Here, we study fold transition between distinct β-barrels by protein engineering and structural biology technique. Here, we discover that the previously reconstructed ancient DPBB sequence could also adopt a β-barrel fold named Double-Zeta β-barrel (DZBB), as a metamorphic protein. The DZBB fold is not found in any modern protein, although its structure shares similarities with RIFT and OB. Furthermore, the reconstructed OB fold could also be converted to the four-stranded SH3 fold by a simple circular permutation. Thus, these ancient β-barrel folds (DPBB, RIFT, OB, and SH3) could be readily interconverted by a few feasible mutations through the missing-link fold, DZBB, indicating their significantly close evolutionary relationships.

To test this assumption, we conducted the reverse engineering by replacing segment 1 of design-13 and design-16 with the 8-amino acid sequence forming the Z-loop of design-2 (the 3rd generation mutants: design-18 (tkoL2_v1.2_Z) and design-19 (mkaL2_v1.2_Z)). SEC and CD experiments demonstrated that both mutants folded and had moderate thermal stabilities. The crystal structures of design-18 and design-19 revealed that they adopt the DZBB fold even without the α1 region (segment 2). These results demonstrated that the segment 1 is sufficient to archive the fold-change from DZBB to OB. Most DNA molecules did not migrate from the well when mixed with the proteins with the stable DZBB fold (design-2, -18, and -19) and RIFT fold (design-3 and -4), indicating that these proteins formed large aggregates with dsDNA. In particular, design-2, -18, -19, -3, and -4 interacted with dsDNA even in high salt conditions (500 mM NaCl). Design-2, -18, -19, -3, and -4 might interact with the phosphate groups in the DNA backbone in a similar way to the sulfate ions in the crystal structures of DZBB.

> GPMPGKKFVARVEEARAEDVGKRVVIIPKGIKVGDVVEVKKV PFOR is a metalloprotein found in several anaerobic microorganisms where it is responsible for the reversible ferredoxin-dependent oxidative decarboxylation of pyruvate. PFOR is a 267 kDa homodimer that contains three [Fe4S4] clusters per monomer. We have used our previous experience with cryo-crystallography to develop a method to prepare cryo-EM grids in an anaerobic chamber and have applied it to solve the structures of apoferritin and the 3 [Fe4S4]-containing pyruvate ferredoxin oxidoreductase (PFOR) at 2.40 Å and 2.90 Å resolution, respectively. [Fe-S] clusters are often sensitive to oxygen-induced degradation, leading to activity loss of the coordinating metalloprotein.

We subsequently prepared cryo-EM grids using our anaerobic setup. As many as 180,868 particles were used to calculate the final 3D reconstruction at an estimated resolution of 2.90 Å by applying the gold standard FSC criterion. Calculation of the local resolution indicates that the protein core, which represents about 83% of the volume of the reconstruction, is at a resolution between 2.75 Å and 3.05 Å, while the most exposed loops at the surface are at lower resolution ranging from 3.05 to 3.55 Å. The most significant difference corresponds to a rotation of 1.6° between monomers when compared to the D. africanus PFOR crystal structures and up to 2.6° when compared to the enzyme from Moorella thermoacetica. The largest disordered region corresponds to the first 14 residues of domain VII (residues 1170–1183), which consists of a domain-swapping extension. In addition, the Cys1195-Cys1212 disulfide bridge, the Ca2+ and Mg2+ ions and the thiamine pyrophosphate (TPP), essential for the protein activity, are clearly visible in the cryo-EM reconstruction. More to the point, the three [Fe4S4] clusters are also perfectly defined in each monomer with high matching density (up to about 15 σ). The four iron and four sulfide atoms are observed in all clusters, and all of the metal ions are bound to their expected cysteine ligands. Only one of the cysteine ligands of the distal [Fe4S4] cluster displays an alternative conformation never seen in the published X-ray structures. The cryo-EM refined model is very similar to previously published PFOR crystal structures, especially for several PFOR features ([Fe4S4] clusters, TPP, disulfide bridges, Ca2+). The only notable difference is an opening of the dimer interface in the latter, which is most likely due to crystal packing.

>[2x]MGKKMMTTDGNTATAHVAYAMSEVAAIYPITPSSTMGEEADDWAAQGRKNIFGQTLTIREMQSEAGAAGAVHGALAAGALTTTFTASQGLLLMIPNMYKISGELLPGVFHVTARAIAAHALSIFGDHQDIYAARQTGFAMLASSSVQEAHDMALVAHLAAIESNVPFMHFFDGFRTSHEIQKIEVLDYADMASLVNQKALAEFRAKSMNPEHPHVRGTAQNPDIYFQGREAANPYYLKVPGIVAEYMQKVASLTGRSYKLFDYVGAPDAERVIVSMGSSCETIEEVINHLAAKGEKIGLIKVRLYRPFVSEAFFAALPASAKVITVLDRTKEPGAPGDPLYLDVCSAFVERGEAMPKILAGRYGLGSKEFSPAMVKSVYDNMSGAKKNHFTVGIEDDVTGTSLPVDNAFADTTPKGTIQCQFWGLGADGTVGANKQAIKIIGDNTDLFAQGYFSYDSKKSGGITISHLRFGEKPIQSTYLVNRADYVACHNPAYVGIYDILEGIKDGGTFVLNSPWSSLEDMDKHLPSGIKRTIANKKLKFYNIDAVKIATDVGLGGRINMIMQTAFFKLAGVLPFEKAVDLLKKSIHKAYGKKGEKIVKMNTDAVDQAVTSLQEFKYPDSWKDAPAETKAEPMTNEFFKNVVKPILTQQGDKLPVSAFEADGRFPLGTSQFEKRGVAINVPQWVPENCIQCNQCAFVCPHSAILPVLAKEEELVGAPANFTALEAKGKELKGYKFRIQINTLDCMGCGNCADICPPKEKALVMQPLDTQRDAQVPNLEYAARIPVKSEVLPRDSLKGSQFQEPLMEFSGACSGCGETPYVRVITQLFGERMFIANATGCSSIWGASAPSMPYKTNRLGQGPAWGNSLFEDAAEYGFGMNMSMFARRTHLADLAAKALESDASGDVKEALQGWLAGKNDPIKSKEYGDKLKKLLAGQKDGLLGQIAAMSDLYTKKSVWIFGGDGWAYDIGYGGLDHVLASGEDVNVFVMDTEVYSNTGGQSSKATPTGAVAKFAAAGKRTGKKDLARMVMTYGYVYVATVSMGYSKQQFLKVLKEAESFPGPSLVIAYATCINQGLRKGMGKSQDVMNTAVKSGYWPLFRYDPRLAAQGKNPFQLDSKAPDGSVEEFLMAQNRFAVLDRSFPEDAKRLRAQVAHELDVRFKELEHMAATNIFESFAPAGGKADGSVDFGEGAEFCTRDDTPMMARPDSGEACDQNRAGTSEQQGDLSKRTKK> HHMLEAKFEEASLFKRIIDGFKDCVQLVNFQCKEDGIIAQAVDDSRVLLVSLEIGVEAFQEYRCDHPVTLGMDLTSLSKILACGNNTDTLTLIADNTPDSIILLFEDTKKDRIAEYSLK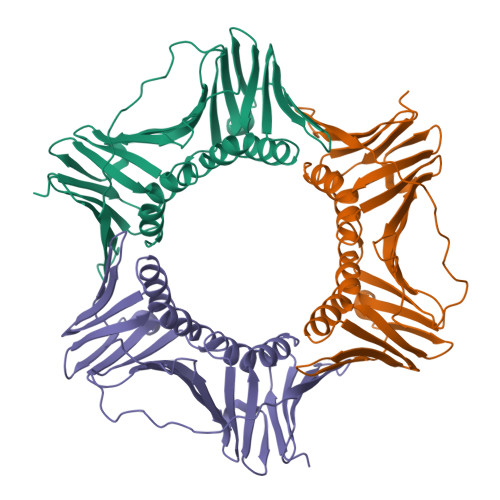LMDIDADFLKIEELQYDSTLSLPSSEFSKIVRDLSQLSDSINIMITKETIKFVADGDIGSGSVIIKPFVDMEHPETSIKLEMDQPVDLTFGAKYLLDIIKGSSLSDRVGIRLSSEAPALFQFDLKSGFLQFFLAPKF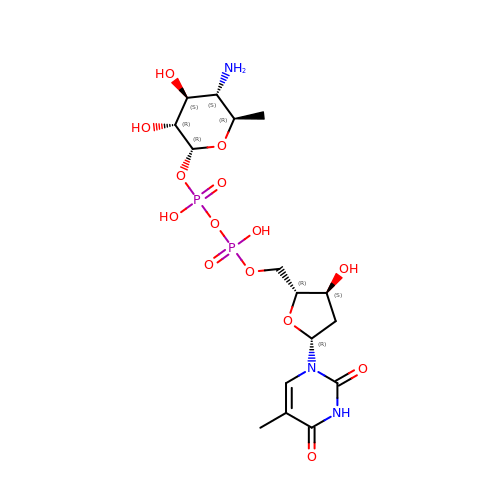dTDP-4-amino-4,6-dideoxyglucose | C16 H27 N3 O14 P2 | UIVJXHWSIFBBCY-LPGAPTBISA-N>MGHHHHHHGSGSTNINLFSSYQLGELELPNRIVMAPLTRSRAGEGNVPHQLNAIYYGQRASAGLIIAEATQVTPQGQGYPHTPGIHSPEQVAGWKLVTDTVHQQGGRIFLQLWHVGRISHPDLQPDGGLPVAPSAIAPKGEVLTYEGKKPYVTPRALDTSEIPAIVEQYRQGAANALAAGFDGVEIHAANGYLIDQFLRDGTNQRTDEYGGAIENRARLLLEVTEAITSVWDSQRVGVRLSPLTTLNGCVDSHPLETFGYVAQALNRFNLSYLHIFEAIDADIRHGGTVVPTSHLRDRFTGTLIVNGGYTREKGDTVIANKAADLVAFGTLFISNPDLPERLEVNAPLNQADPKTFYGGGEKGYTDYPFLAVANK[2x]

To generalize this engineering approach for crystal contacts, a non-ADH-homologous enzyme was selected to apply the established strategies to the Nostoc sp. PCC 1720 ene reductase (NostocER). This oxidoreductase from the old yellow enzyme family (OYE, EC 1.6.99.1) catalyzes the trans-hydrogenations of activated alkenes, demonstrating its industrial relevance as a biocatalyst. As OYEs are strongly dependent on cost-intensive NADPH as a cofactor, Mähler et al. engineered NADH-accepting variants (NostocER1) by exchanging NostocER loop regions at cofactor-binding sites to ER loop regions from Achromobacter sp. JA81 and Acaryochloris marina with a higher NADH affinity. For this study, the NostocER1 Loop1,5 variant (NostocER1-L1,5) was selected as an example protein for the rational introduction of Lys–Glu interactions at crystal contacts to demonstrate the impact of rational single amino acid exchanges on the crystallizability of proteins and enhance protein crystallization.

The NspER1-L1,5 WT and mutants Q204K, Q350K, D352K, and T354K crystallized under the crystallization condition containing 10 g L−1 of purified protein and 150 g L−1 PEG 6000 in the crystallization buffer, whereby the crystal amount was highest, and the crystal size was smallest for mutant T354K, followed by Q204K and D352K. Mutants D352K and T354K crystallizing in the same space group P1211 as the wild type showed, again, an excellent agreement in crystal packing. The distance of 3.5 Å between the carboxy group of E27 and the amino group of mutant T354K indicates the formation of a salt bridge. Distances between the participating functional groups of salt bridges were defined to be ≤4 Å, which could be applied to T354K, explaining its enhanced crystallizability. Introducing a lysine at any of the neighboring NspER1-L1,5 positions Q350, (D352), and T354 led to an interaction with the intermolecular amino acid residue of E25/27. The neighboring NspER1-L1,5 mutants Q350K, D352K, and T354K led to an interaction with intermolecular E25/27 and an increase in crystallizability (Section 3.2, Section 3.3 and Section 3.4), with the strongest impact for T354K. This indicates that introducing electrostatic interactions is not limited to single positions but can also be applied to suitable neighboring amino acid residues, making the approach even more applicable.> HHHHHHHE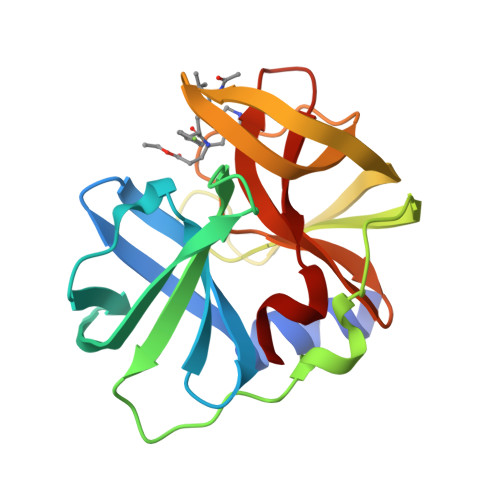FVRALIKRNCHVITTSKGEFNMLGIHDNCAVVPTHAECGDSVTIDGREVRVLKQCILTDTNDTDTEITLLWLDQNEKFRDIRRFIPEHQREWSNMHLATNVTKFPMLDVEVGTVIPYGEVNLSGNPTCRLLKYNYPTKPGQCGGVIANTGNIVAIHVGGNGRVGYGAALLRKYFA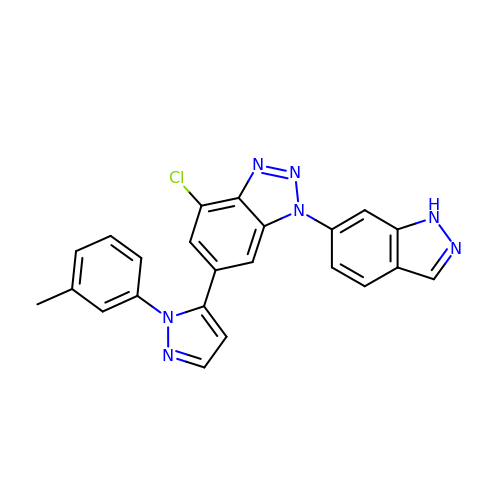4-chloranyl-1-(1~{H}-indazol-6-yl)-6-[2-(3-methylphenyl)pyrazol-3-yl]benzotriazole | C23 H16 Cl N7 | CSVTXOXVXICQEG-UHFFFAOYSA-N>[2x]MHHHHHHKYTVITGASSGIGYETAKLLAGKGKSLVLVARRTSELEKLRDEVKQISPDSDVILKSVDLADNQNVHDLYEGLKEL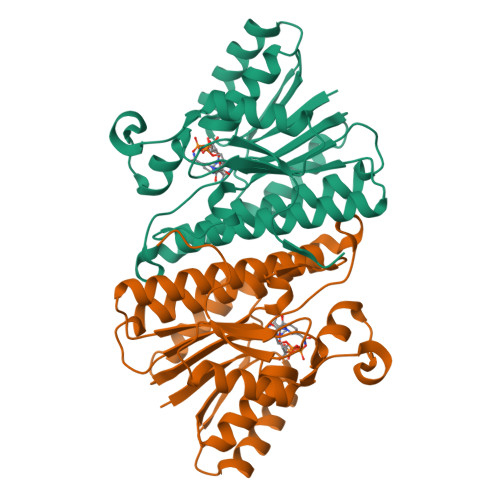DIETWINNAGVGDFDLVQDIELGKIEKMLRLNIEALTILSSLFVRDHHDIEGTTLVNISSLGGYMIVPNAVTYCATKFYVSAYTEGLAQELQKGGAKLRAKVLAPAATETEFVDRARGEAGFDYSKNVKKYHTAAEMAGFLHQLIESDAIVGIVDGETYEFELRGPLFNYAG>UAGCCCC[2x];>[2x]GGGG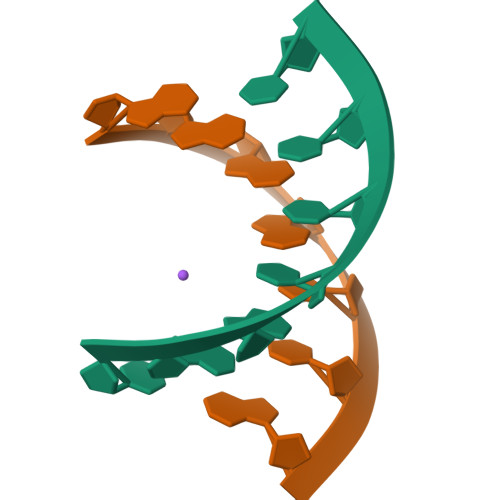CUA>GMENKKMNLLLFSGDYDKALASLIIANAAREMEIEVTIFCAFWGLLLLRDPEKASQEDKSLYEQAFSSLTPREAEELPLSKMNLGGIGKKMLLEMMKEEKAPKLSDLLSGARKKEVKFYACQLSVEIMGFKKEELFPEVQIMDVKEYLKNALESDLQLFI[6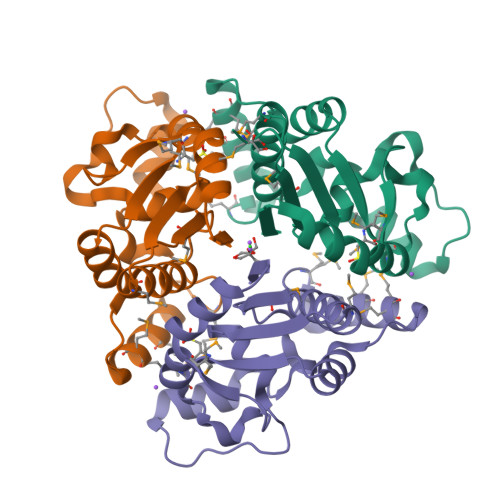x]>[8x]MGVVPQYGGGGNHGGGGNNSGPNSELNIYQYGGGNSALALQTDCRNSDLTITQHGGGNGADVGQGSDDSSIDLTQRGFGNSATLDQWNGKNSEMTVKQFGGGNGAAVDQTASNSSVNVTQCGFGNNATAHQYHHHHHH

Curli, a prototypical functional amyloid formed by IDPs, serves a pivotal role in bacteria. Curli fibrils, widely expressed by Enteric bacteria like Escherichia coli and Salmonella spp., integrate into the extracellular matrix, promoting structural scaffolding, adhesion, and host colonization. The curli system consists of seven proteins encoded by two discrete operons (csgBAC and csgDEFG), which regulate the assembly of a major structural subunit, CsgA, and a minor subunit, CsgB, into curli fibrils. Using cryo-EM, we have shed the first light on the cryo-EM structure of E. coli CsgA fibrils, revealing that the amylogenic regions of CsgA adopt non-centrosymmetric beta-helical structures.

We chose an engineered CsgA with two designed cysteines (A63C and V140C), developed by Balistreri et al., as this selection offers several advantages for structural analysis. The final CsgA fibrils for cryo-EM imaging were formed in 10 mM CAPS buffer with 0.01% Tween 20, pH 10.4, without shaking, and heated at 70°C for 30 min. Acceptable initial 3D models were generated by using box sizes of 218 and 260 pixels. The overall architecture of CsgA fibrils illustrated that seven and eight CsgA subunits could be assigned to the map of 218-pixel and 260-pixel box size, respectively. Interestingly, we also discovered two major spatial arrangements of CsgA fibrils in class 2 (15.5%, 120,429 particles) and class 3 (25.5%, 198,126 particles) of cryo-EM density generated with a 260-pixel box size: a 3-CsgA-fibril bundle and a 2-CsgA-fibril pair. Surprisingly, in the 2-CsgA-fibril pair, two protofilaments made contact through the sides at a specific angle of approximately 34°. This contact likely results from the attraction between uncharged residues on the sides of the fibrils through hydrophobic interactions, while there is repulsion between negatively charged residues on the front and back of the fibrils. The distance between the centers of the two protofilaments was measured at 37.6 Å. Additionally, a less dominant but distinct arrangement, the 3-CsgA-fibril bundles (class 2, 15.5%), also formed at a specific angle (62°, 44°, 74°) and interacted through the sides of the protofilaments. Due to the limit of map quality as a result of preferred orientation, the real resolutions (around 4–6 Å) are lower than the reported values (3.6–3.8 Å) by cryoSPARC, and therefore, the detailed interactions between these molecules within a fibril need to be revealed by further higher-resolution structures.> MMKVFYDSDTTFDAVKDKTIAVIGYGSQGRAQSLN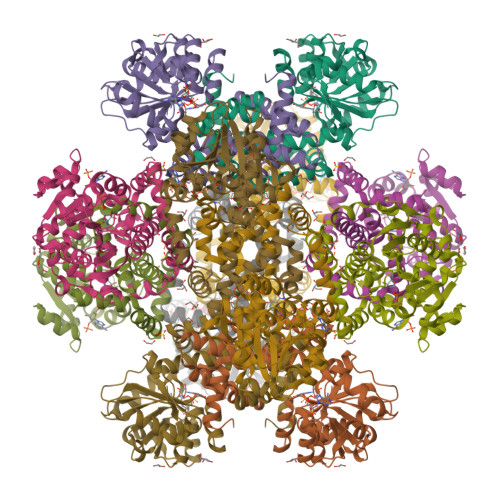MKDSGLKVVVGLRPNGASWNKAKEDGHEVLSIEEAAEKADIIHILIPDEIQGDVYNKQIKPYLKEGKTLSFSHGYNIHYGYIVPPEGVNVVMVAPKSPGAMVRRTYEEGFGVPGLVCVEKDATGDALDIALGMAKGVGLTRAGVIQTTFREETETDLFGEQAVLCGGVTELIKAGFETLVEAGYSPEMAYFETCHELKLIIDLIYQKGFAGMWNDVSNTAEYGGLTRRSRVINEQSRQEMRKILKEIQDGRFTKEWALENISGKAHLNSMRRIESELLIEEVGAKLRKMCGLQKD>[8x]MKSNGCRYGTHRVIEPKGVLPQPAKILNNDMSEIWDNEMLIDVIRLNIDSASFHQIKNKLIAQGHQDLEKAFAEHAIELTNRTGKHKNEDTGSGGMFIGRVAAIGDKFEMKEE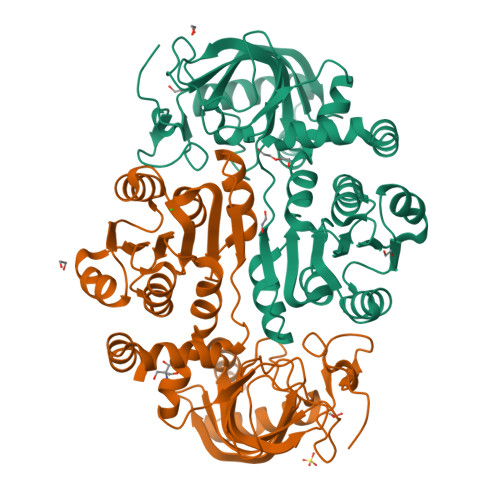VKVGDKIASLVSLSLTPLKINKVKKVLLDKDQMEIEGQAILFSSGVYAKLPDDLDENLALSVLDVAGAPAQVERLVKPDDTVVIIGANGKSGILCNAVAKERAGICGKVIGVVRNENYIPTCKATGCDEVILAQATDAITIQKEVSRLTNGKMADVVINVVNTEDTELPSIMAAKDRGMVYFFSMATSFTKAALGAEGIGADVDMMIGNGYAHHHSEIALDLLRRNSVLMKIFKERYAEHHHHHH> INLPGPMSLIDNTKGQLVVNPEALKILSAITQPVVVVAIVGLYRTGKSYLMNKLAGKKNGFSLGSTVKSHTKGIWMWCVPHPKKPEHTLVLLDTEGLGDIEKGDNENDSWIFALAILLSSTFVYNSMGTINQQAMDQLHYVTELTDRIKANSSPGNNSVDDSADFVSFFPAFVWTLRDFTLELEVDGEPITADDYLELSLKLRKGTDKKSKSFNDPRLCIRKFFPK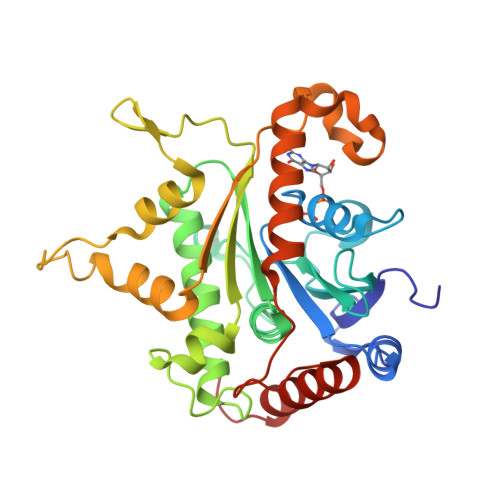RKCFVFDWPAPKKYLAHLEQLKEEELNPDFIEQVAEFCSYILSHSNVKTLSGGIPVNGPRLESLVLTYVNAISSGDLPC>GSHMAKHEQILVLDPPSDLKFKGPFTDVVTTNLKLQNPSDRKVCF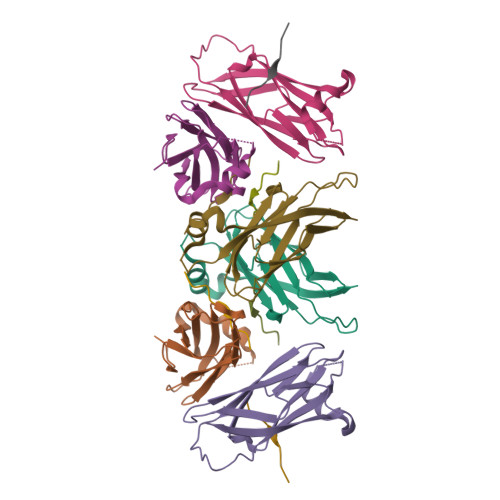KVKTTAPRRYCVRPNSGVIDPGSIVTVSVMLQPFDYDPNEKSKHKFMVQTIFAPPNISDMEAVWKEAKPDELMDSKLRCVFEM[6x];>[6x]SEDEFYDALS(S)-Flurbiprofenoyl-CoA | C36 H47 F 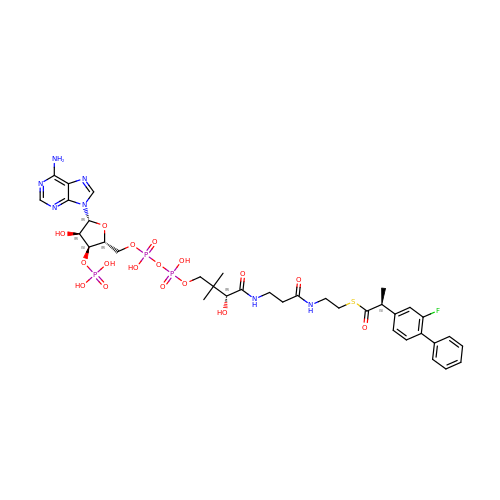N7 O17 P3 S | GFOGIIXIXKGLHP-PJHIEXQGSA-N>[2x]AERIVTIGGDVTEIAYALGAGDEIVARDSTSQQPQAAQKLPDVGYMRTLNAEGILAMKPTMLLVSELAQPSLVLTQIASSGVNVVTVPGQTTPESVAMKINAVATALHQTEKGQKL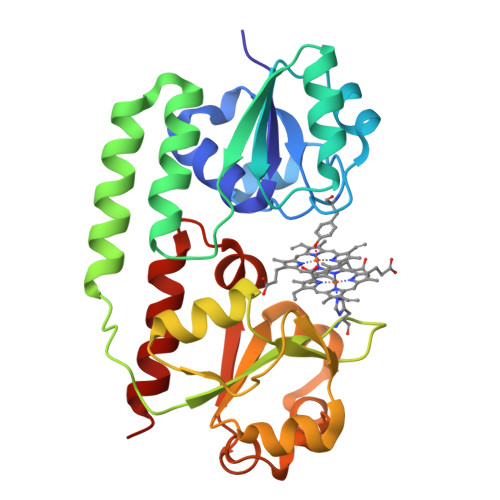IEDYQQRLAAVNKTPLPVKVLFVMSHGGLTPMAAGQNTAADAMIRAAGGSNAMQGFSRYRPLSQEGVIASAPDLLLITTDGVKALGSSENIWKLPGMALTPAGKHKRLLVVDDMALLGFGLETPQVLAQLREKMEQMQ Adseverin (also known as scinderin) is a member of the gelsolin superfamily of Ca2+-dependent actin-binding proteins, which regulate cytoskeletal dynamics by severing, bundling and capping of actin filaments. Adseverin is composed of six GH domains (A1–A6) and shares 60% overall sequence identity with gelsolin (G1–G6). Adseverin was first identified in chromaffin cells of bovine adrenal medulla, where it acts as an actin depolymerizing agent that disassembles the cortical network of actin filaments in response to bursts of intracellular calcium, leading to exocytosis of secretary vesicles. Crystallographic studies revealed that these binding events involve the association of eight calcium ions, six of which bind at a conserved site on each domain (type II), whereas the remaining two are also stabilized by contacts with actin (type I; refs 17, 18, 19, 20). Both proteins are able to sequester two monomers of actin, as well as sever and cap actin filaments through distinct Ca2+-induced domain rearrangements of the two halves of the molecule.

We crystallized A1–A3 in the presence of EGTA, revealing a compact auto-inhibited structure similar to the conformational state observed in inactive full-length gelsolin. Purified recombinant A1–A3, supplemented with 5 mM EGTA, crystallized in space group C2 and its structure was solved by molecular replacement using the structure of G1–G3 excised from inactive full-length gelsolin as the search model and refined to a resolution of 2.9 Å. Each domain adopts the classic GH fold, which is organized around a central five-stranded mixed β-sheet sandwiched between a long α-helix running approximately parallel to the strands, and a shorter α-helix running approximately perpendicular to the strands. The domains adopt the compact arrangement characteristic of inactive gelsolin, with A1 sandwiched between A2 and A3. In this inactive conformation, the long α-helix of A3 is kinked to enable the formation of the A1/A3 latch, resulting in the masking of the major actin-binding interface on A1. The structure appears to be relatively rigid, with B-factors indicating that flexibility is limited mainly to the extended A2A3 linker and the short α-helices of A1 and A2. The inactive forms of A1–A3 (iA1–A3) and G1–G3 (iG1–G3) are highly similar with an overall root mean squared deviation (r.m.s.d.) in Cα positions of 1.19 Å over 337 aligned residues, highlighting the structural conservation between gelsolin and adseverin. The iA1–A3 crystal lattice is stabilized by a number of crystal contacts, including a relatively large packing interface of ∼1,518 Å2. Interestingly, comparisons with full-length gelsolin show that this interface largely buries the surfaces in iA1–A3 that bind the C-terminal half of the molecule, suggesting that the crystal environment partially mimics the inactive full-length protein.

>YHEEFARAGKQAGLQVWRIEKLELVPVPQSAHGDFYVGDAYLVLHTAKTSRGFTYRLHFWLGKECSQDESTAAAIFTVQMDDYLGGKPVQNRELQGYESNDFVSYFKGGLKYKAGGVASGLNHVLTNDLTAKRLLHVKGRRVVRATEVPLSWDSFNKGDCFIIDLGTEIYQWCGSSCNKYERLKANQVATGIRYNERKGRSELIVVEEGSEPSELIKVLGEKPELPDGGDDDDIIADISNRKMAKLYMVSDASGSMRVTVVAEENPFSMAMLLSEECFILDHGAAKQIFVWKGKDANPQERKAAMKTAEEFLQQMNYSKNTQIQVLPEGGETPIFKQFFKDWRD[2x]>APTPAQMPSPTSFSDSIKQLAAETLPKYMQQLN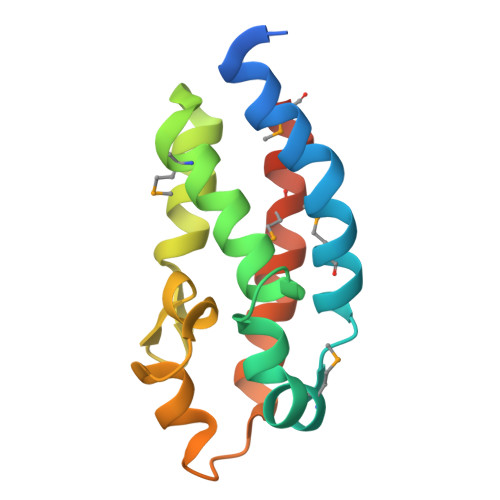SLDAEMLQKNHDQFATGSGPLRGSITQCQGLMQFCGGELQAEASAILNTPVCGIPFSQWGTIGGAASAYVASGVDLTQAANEIKGLAQQMQKLLSLMHHHHHH[2x]(2~{R})-~{N}-(2-azanylideneethyl)-2-[2-(3-methyl-1,2-oxazol-5-yl)ethanoylamino]-3-(4-pyridin-2-ylpiperazin-1-yl)sulfonyl-propanamide | 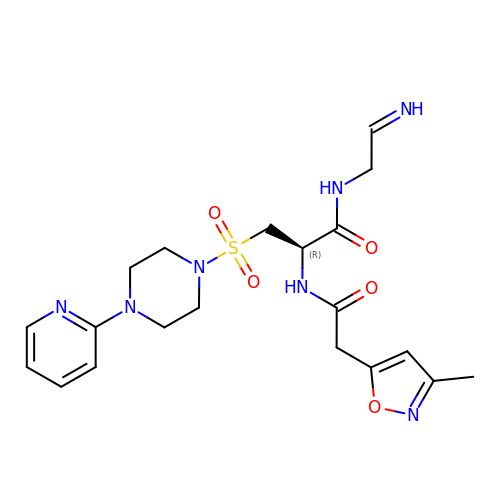C20 H27 N7 O5 S | RJJWMSGSKPHRAN-NEEXXPDWSA-N6-chloro-N~4~-cyclopropyl-N~4~-[(thiophen-2-yl)methyl]pyrimidine-2,4-diamine | C12 H13 Cl N4 S | 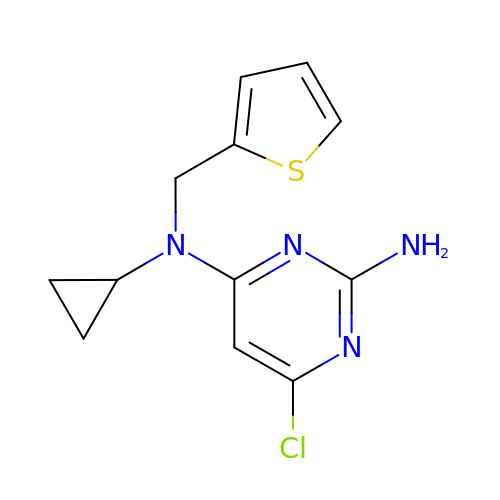PDWZXKSZLRVSEH-UHFFFAOYSA-N>[4x]MGSSHHHH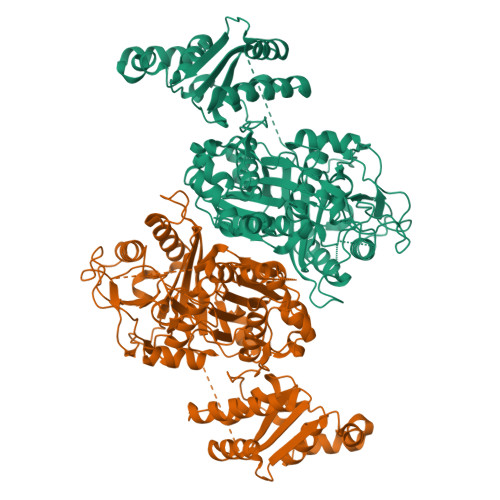HHSSGLVPRGSSDRPEDAIAIVGMSGRYPGARNVREYWDNLVHARNAIRDIPTSRWDVDKYYDPVLNKKGKVYCKSMGMLDDIEHFDPLFFNIPPSEAELMDPQHRIFLQEGYKAFEDAGYNARTLNEKKCGVYLGIMSNEYGVMLNRQSRANATGNSFAIAAARIPYFLNLKGPAIPIDTASSSSLVGTHLARQALINKEIDMALVGGVSLYLTPESYMSMCEAGMLSPDGQCKAFDNGANGFVPGEGAGALVLKRLKDAEADRDHIYGIIIGSGINQDGKTNGITAPSAKSQMDLERDIYETYGIHPESISYVEMHGTGTKQGDPIELEALSTVFQEKTDKKQFCAIGSVKSNIGHTSAAAGVAGVQKVLLCMNHKTLVPTLNFTTPNEHFEFEHSPLYVNTELKPWETADGKPRRACVSSFGYSGTNAHIVIEEYQPEKRNDRLTKQHRSALFVLSAKKEKQLKAYAEAMKDFVTSNEDIDLEDMAYTLQTGREAMDYRMAFLADSREMLIKALDDYLAEMPNGSIFAAHVKTKKSEIKLFETDHDAKALLQTWIEKKRLEKVAELWVKGLQIDWNKLYGEYTPRRISLPAYPFAEEYYWLPTQEG>[3x]MPEGPELHLASQFVNEACRALVFGGCVEKSSVSRNPEVPFESSAYRISASARGKELRLILSPLPGAQPQQEPLALVFRFGMSGSFQLVPREELPRHAHLRFYTAPPGPRLALCFVDIRRFGRWDLGGKWQPGRGPCVLQEYQQFRENVLRNLADKAFDRPIC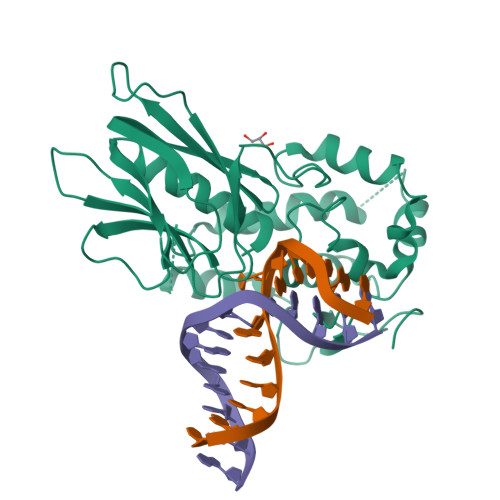EALLDQRFFNGIGNYLRAEILYRLKIPPFEKARSVLEALQQHRPSPELTLSQKIRTKLQNPDLLELCHSVPKEVVQLGGKGYGSESGEEDFAAFRAWLRCYGMPGMSSLQDRHGRTIWFQGDPGPLAPKGRKS> RPASELLKYLT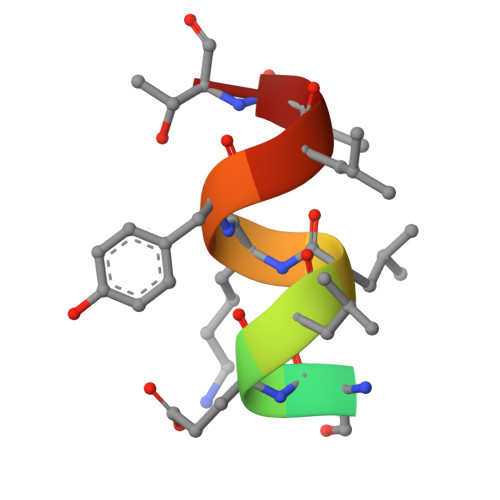T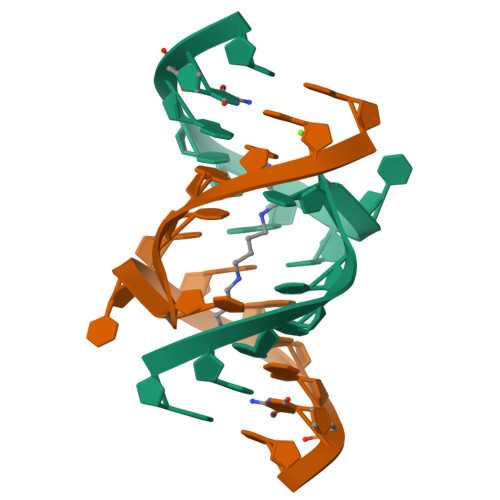>[2x]GGUAUUUCGGUACC> MPLCASPVRLQLCRTPSV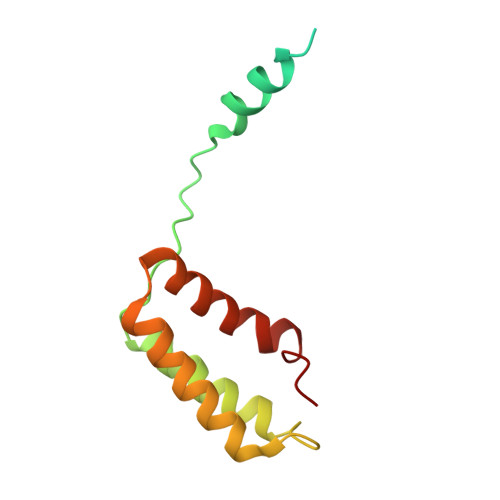LGAGGKWWKEGPPDYTRANRRRMELEQQRIESSQHLPPIEPTAEQACHLYRRLLKEGYKTLVVTDKDFYRRKVRYELEVTSRQTSSRVRGIMFEKGHWMLENKLGGII> MPFCTSTPEPEAQSTEQSLTCEGQIISGTSVDASDLVTGNEIGEQQLISGDAYVGAQQTGCLPTSPRFNQTGNVQSMGFKNTNQPEQNFAPGEVMPTDFSIQTPARSAQNRITGNDIAPSGRITGPGMLATGLITGTPEFRHAARELVGSPQPMAMAMANRNKAAQAPVVQPEVVATQEKPELVCAPRSDQMDRVSGEGKERC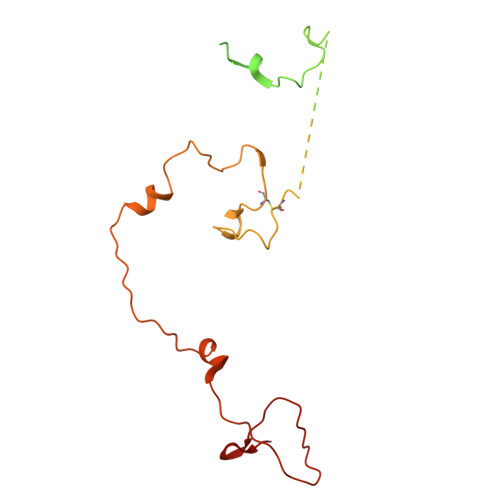HITGDDWSVNKHITGTAGQWASGRNPSMRGNARVVETSAFANRNVPKPEKPGSKITGSSGNDTQGSLITYSGGARG> HEELA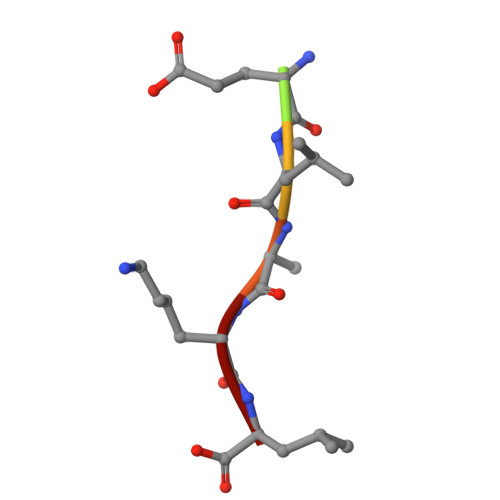KL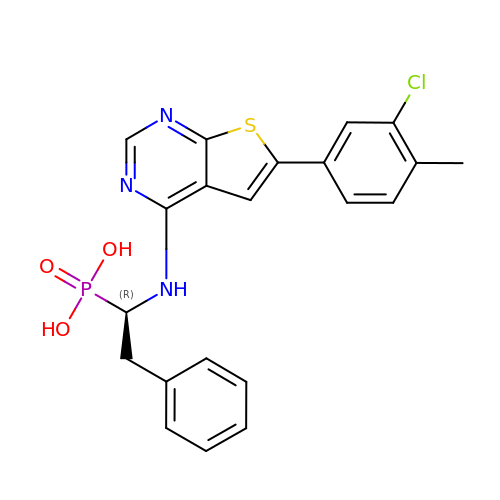[(1R)-1-{[6-(3-chloro-4-methylphenyl)thieno[2,3-d]pyrimidin-4-yl]amino}-2-phenylethyl]phosphonic acid | C21 H19 Cl N3 O3 P S | FHHLLOYGUMAOOP-LJQANCHMSA-N>MRGSHSGAQGLLAAQKARGLFKDFFPETGTKIELPELFDRGTASFPQTIYCGFDPTADSLHVGHLLALLGLFHLQRAGHNVIALVGGATARLGDPSGRTKEREALETERVRANARALRLGLEALAANHQQLFTDGRSWGSFTVLDNSAWYQKQHLVDFLAAVGGHFRMGTLLSRQSVQLRLKSPEGMSLAEFFYQVLQAYDFYYLFQRYGCRVQLGGSDQLGNIMSGYEFINKLTGEDVFGITVPLITSTTGAKLGKSAGNAVWLNRDKTSPFELYQFFVRQPDDSVE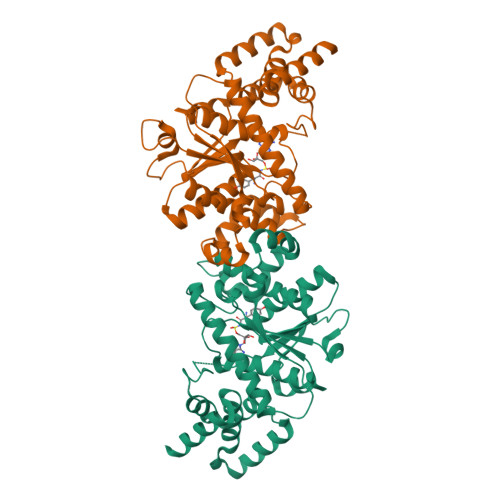RYLKLFTFLPLPEIDHIMQLHVKEPERRGPQKRLAAEVTKLVHGREGLDSAKRCTQALYHRSHHHHHH[2x]> MG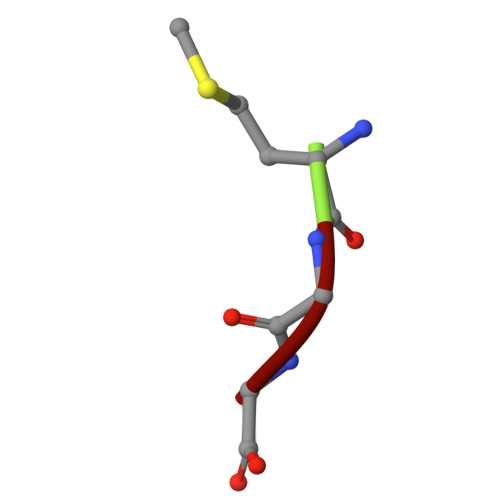G> SIVLEPIYWNSSNSKFLPGQGLVLYPQIGDKLDIICPKVDSKTVGQYEYYKVYMVDKDQADRCTIKKENTPLLNCAKPDQDIKFTIKFQEFSPNLWGLEFQKNKDYYIISTSNGSLEGLDNQE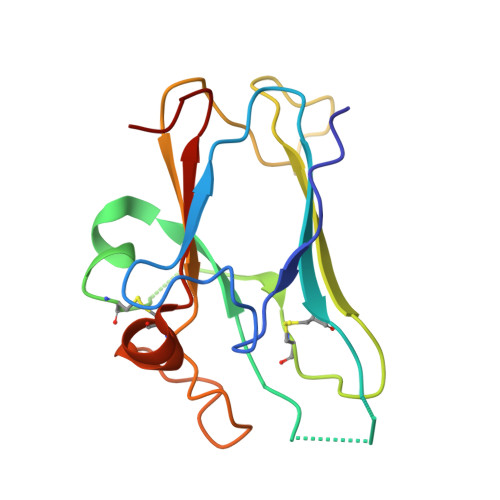GGVCQTRAMKILMKVGQDAS> QYSPNTQQGRTSIVHLFEWRWVDIALECERYLAPKGFGGVQVSPPNENVAIYNPFRPWWERYQPVSYKLCTRSGNEDEFRNMVTRCNNVGVRIYVDAVINHMCGNAVSAGTSSTCGSYFNPGSRDFPAVPYSGWDFNDGKCKTGSGDIENYNDATQVRDCRLTGLLDLALEKDYVRSKIAEYMNHLIDIGVAGFRLDASKHMWPGDIKAILDKLHNLNSNWFPAGSKPFIYQEVIDLGGEPIKSSDYFGNGRVTEFKY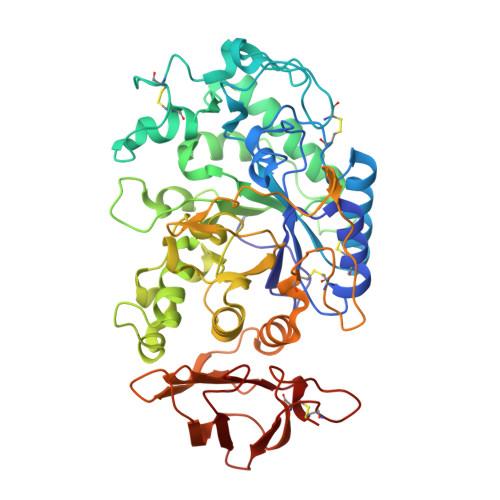GAKLGTVIRKWNGEKMSYLKNWGEGWGFVPSDRALVFVDNHDNQRGHGAGGASILTFWDARLYKMAVGFMLAHPYGFTRVMSSYRWPRQFQNGNDVNDWVGPPNNNGVIKEVTINPDTTCGNDWVCEHRWRQIRNMVIFRNVVDGQPFTNWYDNGSNQVAFGRGNRGFIVFNNDDWSFSLTLQTGLPAGTYCDVISGDKINGNCTGIKIYVSDDGKAHFSISNSAEDPFIAIHAESKL>[4x]GGVMSLLCVGVKKAKFDGAQEKFNTYVTLKVQNVKSTTIAVRGSQPSWEQDFMFEINRLDLGLTVEVWNKGLIWDTMVGTVWIP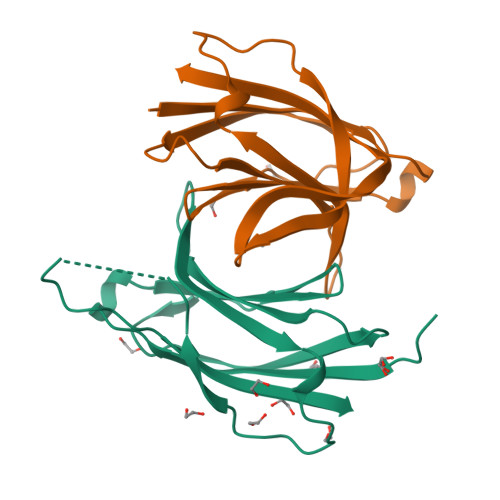LRTIRQSNEEGPGEWLTLDSQAIMADSEICGTKDPTFHRILLDAHFE> MAYTTFSQTKNDQLKEPMFFGQPVNVARYDQQKYDIFEKLIEK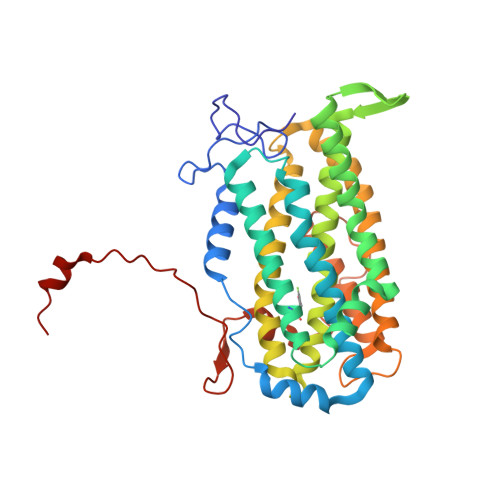QLSFFWRPEQVDVSRDRIDYQALPEHEKHIFISNLKYQTLLDSIQGRSPNVALLPLISIPELETWVETWAFSETIHSRSXTHIIRNIVNDPSVVFDDIVTNEQIQKRAEGISSYYDELIEMTSYWHLLGEGTHTVNGKTVTVSLRELKKKLYLCLMSVNALEAIRFYVSFACSFAFAERELMEGNAKIIRLIARDEALHLTGTQHMLNLLRSGADDPEMAEIAEECKQECYDLFVQAAQQEKDWADYLFRDGSMIGLNKDILCQYVEYITNIRMQAVGLDLPFQTRSNPIPWINTWLVSDNVQVAPQEVEVSSYLVGQIDSEVDTDDLSNFQL>[4x]GSHMAHAMENSWTISKEYHIDEEVGFALPNPQENLPDFYNDWMFIAKHLPDLIESGQLRERVEKLNMLSIDHLTDHKSQRLARLVLGCITMAYVWGKGHGDVRKVLPRNIAVPYCQLSKKLELPPILVYADCVLANWKKKDPNKPLTYENMDVLFS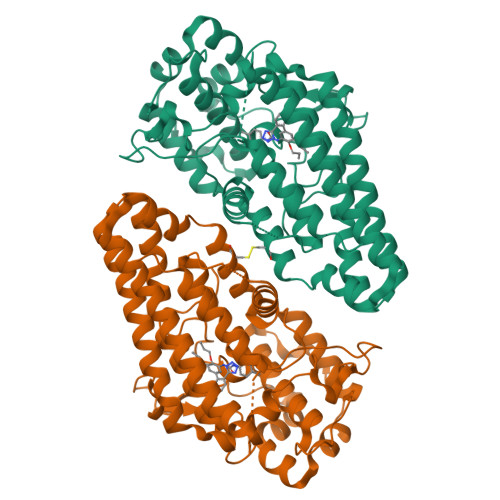FRDGDCSKGFFLVSLLVEIAAASAIKVIPTVFKAMQMQERDTLLKALLEIASCLEKALQVFHQIHDHVNPKAFFSVLRIYLSGWKGNPQLSDGLVYEGFWEDPKEFAGGSAGQSSVFQCFDVLLGIQQTAGGGHAAQFLQDMRRYMPPAHRNFLCSLESNPSVREFVLSKGDAGLREAYDACVKALVSLRSYHLQIVTKYILIPASQQPKENKTSEDPSKLEAKGTGGTDLMNFLKTVRSTTEKSLLKEG> 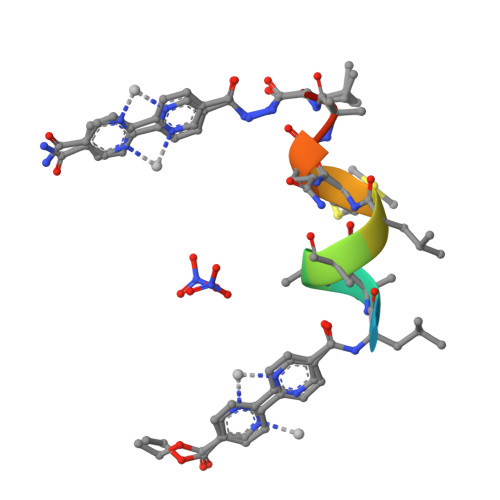XLAAALMQALX>SGSVKIRNVTSNHRASDTVVCEGRPQVLNGRFMYGPLDVVTLTGEKVDVYVMTQPLSGKWIHFGTEVTNSSGRLTFPVPSERALGIGVYPVRMVVRGDHTYAECCLTVVSRGTEAVVFSIDGSFTASVSIMGSDPKVRAGAVDVVRHWQDSGYLIVYVTGRPDMQKHRVVAWLSQHNFPHGVVSFCDGLTHDPL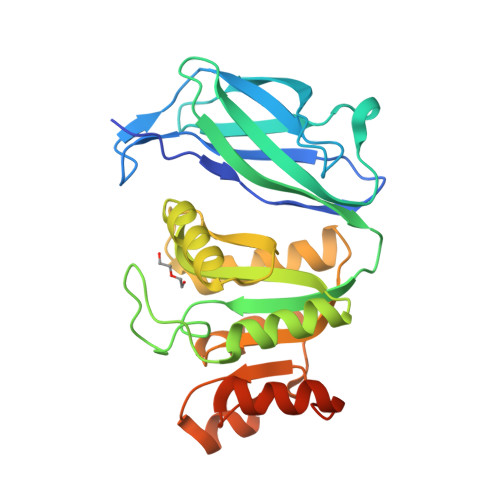RQKAMFLQSLVQEVELNIVAGYGSPKDVAVYAALGLSPSQTYIVGRAVRKLQAQCQFLSDGYVAHLGQLEAGSHSHAPSGPPRAALAKSS[3x]> STVTLPETLLFVSTLDGSLHAVSKRTGSIKWTLKEDPVLQVPTHVEEPAFLPDPNDGSLYTLGSKNNEGLTKLPFTIPELVCASPSRSSDGILYMGKKQDIWYVIDLLTGEKQQTLSSAFADSLSPSTSLLYLGRTEYTITMYDTKTRELRWNATYFDYAASLPEDDVDYKMSHFVSNGDGLVVTVDSESGDVLWIQNYASPVVAFYVWQREGLRKVMHINVAVETLRYLTFMSGEVGRITKWKYPFPKETEAKSKLTPTLYVGKYSTSLYASPSMVHEGVAVVPRGSTLPLLEGPQTDGVTIGDKGESVITPSTDVKFDPGLKSKNKLNYLRNYWLLIGHHETPLSASTKMLERFPNNLPKHRENV

In eukaryotes, the endoplasmic reticulum (ER) is the central organelle for the synthesis of proteins destined for secretion and membrane insertion. To ensure that the environment for productive protein maturation is maintained, both folding capacity and the inward flux of newly synthesised proteins are regulated by a pervasive negative feedback signalling pathway, the unfolded protein response (UPR). IRE1, conserved in all eukaryotes and therefore the best-studied UPR transducer, detects ER stress via its luminal domain (IRE1LD), initiating dimerisation-dependent autophosphorylation of its cytosolic domain. An alternative hypothesis posits that IRE1 is repressed by interacting with a major component of the ER folding machinery, the heat-shock protein (Hsp70) chaperone BiP.

The luminal domain of the broadly expressed alpha isoform of human IRE1 (hIRE1αLD) also crystallises as a dimer, with an overall architecture similar to the yeast protein, however, barring conformational changes, the MHC-like groove is too narrow to accommodate a peptide. Hence, it has been proposed that the structure of Zhou et al. (2006) represents a ‘closed’ conformation of the peptide-binding groove that can shift towards an ‘open’ state to allow peptide binding. To confirm these observations, we made use of an alternative assay reporting on IRE1LD’s dimerisation status. To this end, we employed a modified IRE1LD Q105C that forms a disulphide across the dimer interface, creating a covalently stabilised dimer when placed in oxidising conditions and the aforementioned dimerisation-compromised versions of the IRE1LD (W125A and P108A). Differential scanning fluorimetry (DSF) revealed that the melting temperature (Tm) of disulphide-linked IRE1LD Q105C SS was ~10 °C higher than the Tm the wild-type protein, a Tm difference that was effaced by reduction of the dimer-stabilising disulphide. To gain insight into the mode of MPZ-N binding to IRE1LD we made further use of the disulphide-linked IRE1LD Q105C SS. The crystallised IRE1LD Q105C SS dimer proved identical in structure to the wild-type protein (root-mean squared deviation (RMSD) of 0.46 Å over 227 Cα atoms) except for the presence of a conspicuous density corresponding to a C105-C105 trans-protomer disulphide, thereby locking the proposed binding groove in the ‘closed’ conformation. Nonetheless, a fluorescence polarisation binding assay, using FAM-labelled MPZ-N, showed that binding to the IRE1LD was not compromised by the disulphide, leading us to conclude that MPZ-N does not obligatorily bind within the proposed MHC-like groove of the IRE1LD. Our findings do not support the notion that this peptide specifically engages the MHC-like groove traversing the dimer interface, as a disulphide, crystallographically proven to lie across this groove, thereby locking the helices in a ‘closed’ conformation, had no effect on the binding of MPZ-N to IRE1LD.> SNAMKAIIKEDVQASLE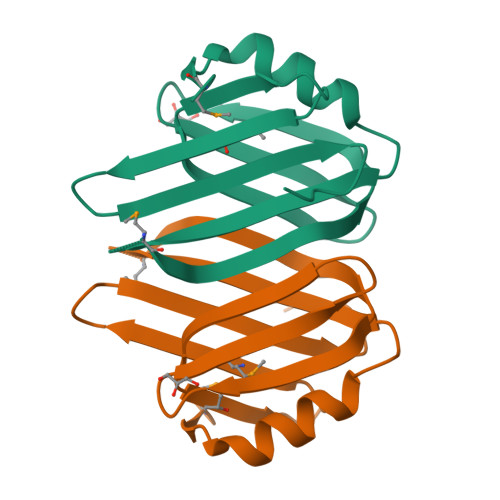RYADRPVYIHLETTTGSYSAHLNEKNMTVVAYIRNAKVTYHQAKIKGNGPYRVGLKTEEGWIYAEGLTEYTVDEENRLLMAGHLPGGKLAISLQISEKPFTV> MADSELQLVEQRIRSFPDFPTPGVVFRDISPVLKDPASFRAAIGLLARHLKATHGGRIDYIAGLDSRGFLFGPSLAQELGLGCVLIRKQGKLPGPTLWASYSLEYGKAELEIQKDALEPGQRVVVVDDLLATGGTMNAACELLGRLQAEVL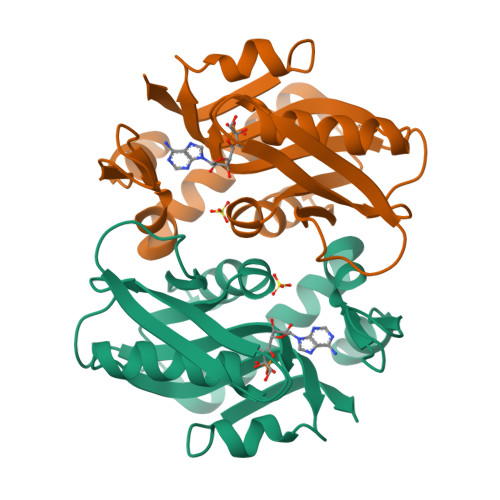ECVSLVELTSLKGREKLAPVPFFSLLQYE> GSVLCSTPTINIPASPFMQKLGFGTGVNVYLMKRSPRGLSHSPWAVKKINPICNDHYRSVYQKRLMDEAKILKSLHHPNIVGYRAFTEANDGSLCLAMEYGGEKSLNDLIEERYKASQDPFPAAIILKVALNMARGLKYLHQEKKLLHGDIKSSNVVIKGDFETIKICDVGVSLPLDENMEVTDPEACYIGTEPWKPKEAVEENGVITDKAD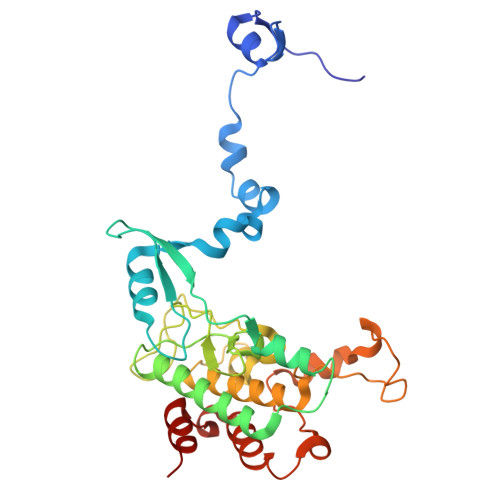IFAFGLTLWEMMTLSIPHINLSNDDDDEDKTFDESDFDDEAYYAALGTRPPINMEELDESYQKVIELFSVCTNEDPKDRPSAAHIVEALEAA> RSMAAEVYFGDLELFEPFDHPGESIPKPVHTRFKDDDGDEEDENGVGDAELRERLRQCEETIEQLRAENQELKRKLNILTRPSGILVNDTKLDGPILQILFMNNAISKQYHQEIEEFVSNLVKRFEEQQKNDVEKTSFNLLPQPSSIVLEEDHKVEESCAIKNNKEAFSVVGSVLYFTNFCLDKLGQPLLNENPQLSEGWEIPKYHQVFSHIVSLEGQEIQVKAKRPKPHCFNCGSEEHQMKDCPMPRNAARISEKRKEYMDACGEANNQNFQQRYHAEEVEERFGRFKPGVISEELQDA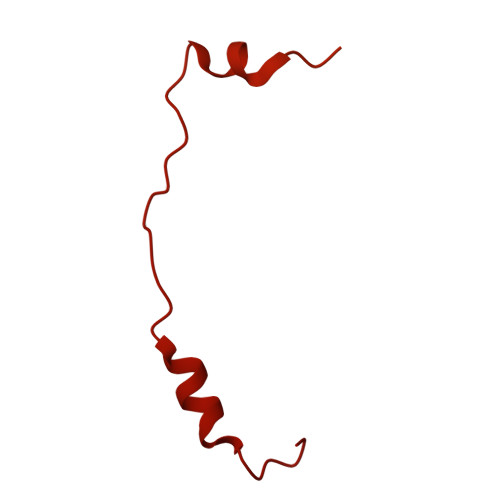LGVTDKSLPPFIYRMRQLGYPPGWLKEAELENSGLALYDGKDGTDGETEVGEIQQNKSVTYDLSKLVNYPGFNISTPRGIPDEWRIFGSIPMQACQQKDVFANYLTSNFQAPGVKSGNKRSSSHSSPGSPKKQKNESNSAGSPADMELDSDMEVPHGSQSSESFQFQPPLPPDTPPLPRGTPPPVFTPPLPKGTPPLTPSDSPQTRTGSGAVDEDALTLEELEEQQRRIWAALEQAESVNSDSDVPVDTPLTGNSVASSPCPNELDLPVPEGKTSEKQTLDEPEVPEIFTKKSEAGHASSPDSEVTSLCQKEKAELAPVNTEGALLDNGSVVPNCDISNGGSQKLFPADTSPSTATKIHSPIPDMSKFATGITPFEFENMAESTGMYLRIRSLLKNSPRNQQKNKKASE>[2x]MVLYFIGLGLYDERDITVKGLEIAKKCDYVFAEFYTSLMAGTTLGRIQKLIGKEIRVLSREDVELNFENIVLPLAKENDVAFLTPGDPLVATTHAELRIRAKRAGVESYVIHAPSIYSAVGITGLHIYKFGKSATVAYPEGEWFPTSYYDVIKENAERGLHTLLFLDIKAEKRMYMTANEAMELLLKVEDMKKGGVFTDDTLVVVLARAGSLNPTIRAGYVKDLIREDFGDPPHI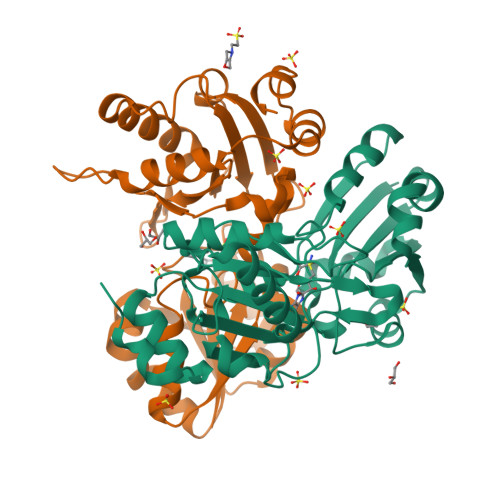LIVPGKLHIVEAEYLVEIAGAPREILRVNV>ELICIVQRVNESFSLHSGFGGNVYSMKTEPMTGFTNVTKGASVINQKDWIGFGDARTDLTNDQFPASSDVPLAVAKKFRSLSGASLMLSAFGPPGKVDYLYQGCGKEKVFYEGVNWSPEAGIDCFGSNWTQTKKDFYSRIYEAARSSTCMTLVNSLDTKISSTTATAGTASSCSSSWMKSPLWYAESSVNPGAKPQVCGTEQSATFTLPTSFGIYKCNKHVVQLCYFVYENKAKFNTFGCGDYYQNYYDGNGNLIGGMDNRVAAYRGIANAGVKIECPSKIL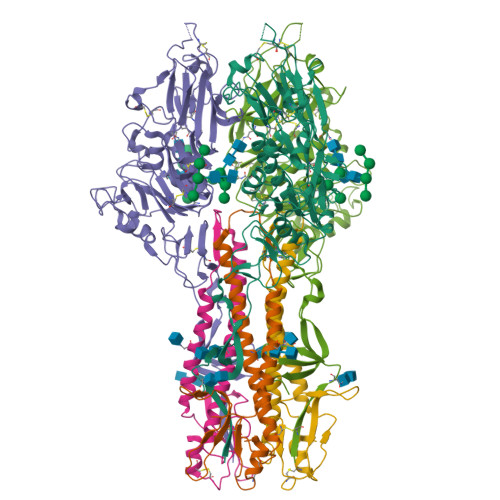NPGTYSIKSTPRFLLVPKRSYCFDTDGGYPIQVVQSEWSASRRSDNATEEACLQTEGCIFIKKTTPYVGEAADNAGDIEMRQLLSGLGNNDTVCVSQSGYTKGETPFVKDYLSPPKYGRCQLKTDSGRIPTLPSGLIIPQAGTDS[2x];>IFGIDDLIFGLLFVGFVAGGVAGGYFWGRSNGGGGGASVSSTQAGFDKIGKDIQQLRNDTNAAIEGFNGRIAHDEQAIKNLAKEIEDARAEALVGELGIIRSLIVANISMNLKESLYELANQITKRGGGIAQEAGPGCWYVDSENCDASCKEYIFNF[2x]> DGIPSFVTAGKCASVANQDNFDLRRYAGRWYQTHIIENAYQPVTRCIHSNYEYSTNDYGFKVTTAGFNPNDEYLKIDFKVYPTKEFPAAHMLIDAPSVFAAPYEVIETDYETYSCVYSCITTDNYKSEFAFVFSRT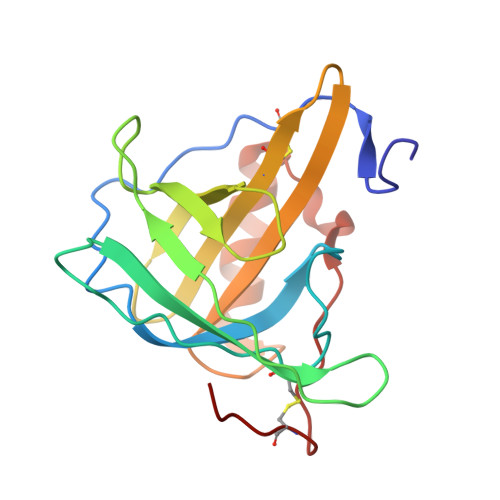PQTSGPAVEKTAAVFNKNGVEFSKFVPVSHTAECVYRA> MVVRFQSSMGRSLKRVDSDDLNVKGLVLATVSKINYKYQSVEVKVNNLTLGSRIGDDGSLAVPYPKSFIGRTPEGSVFGTKPLITEGSVVLIGFLNDDINSPIILSVYGDNEQNKMINTNPLDGGKFDTESVYKYSSSLYEILPSLNYKYDDGEGTSIRTYNGKSFFSMTSGEEEKPQATDFYTGTEYQDLFTSYYGNKTLIEPRIQKAPNMLFKHQGVFYDDGTPDNHITTLFISERGDIRASVLNTETQKRTTQEMSSDGSYRVIKQDDDLMLDEAQVWIEYGISEDNKFYIKNDKHKFEFTDEGIYIDDKPMLENLDE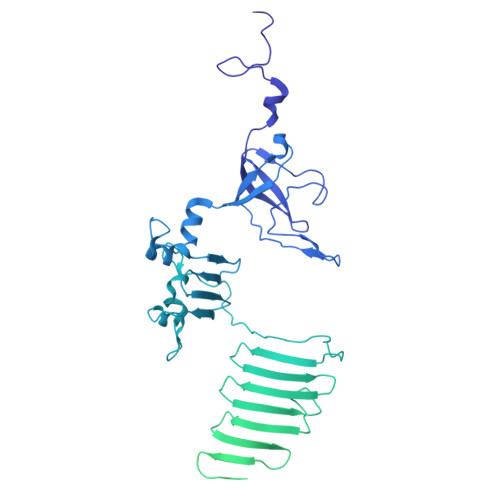SIAEAMKNLNEIQKELDDINYLLKGVGKDNLEELIESTKESIEASKKATSDVNRLTTQIAEVSGRTEGIITQFQKFRDETFKDFYEDASTVINEVNQNFPTMKTDVKTLKTKVDNLEKTEIPNIKTRLTELENNNNNADKIISDRGEHIGAMIQLEENVTVPMRKYMPIPWSKVTYNNAEFWDSNNPTRLVVPKGITKVRVAGNVLWDSNATGQRMLRILKNGTYSIGLPYTRDVAISTAPQNGTSGVIPVKEGDYFEFEAFQDSEGDRQFRADPYTWFSIEAIELETETMEKDFMLIGHRGATGYTDEHTIKGYQMALDKGADYIELDLQLTKDNKLLCMHDSTIDRTTTGTGKVGDMTLSYIQTNFTSLNGEPIPSLDDVLNHFGTKVKYYIETKRPFDANMDRELLTQLKAKGLIGIGSERFQVIIQSFARESLINIHNQFSNIPLAYLTSTFSESEMDDCLSYGFYAIAPKYTTITKELVDLAHSKGLKVHAWTVNTKEEMQSLIQMGVDGFFTNYLDEYKKI>GPMPGEIRPTIGQQMETGDQRFGDLVFRQLAPNVWQHTSYLDMPGFGAVASNGLIVRDGGRVLVVDTAWTDDQTAQILNWIKQEINLPVALAVVTHAHQDKMGGMDALHAAGIATYANALSNQLAPQEGMVAAQHSLTFA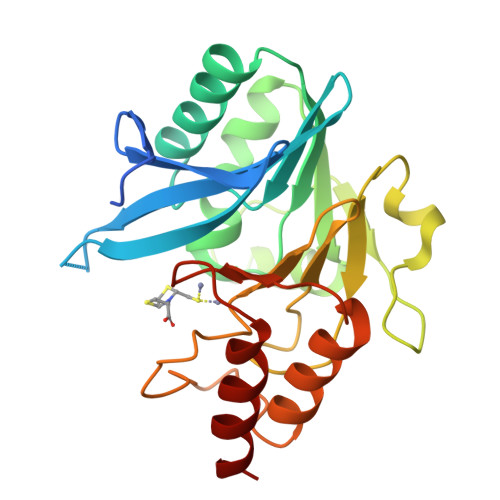ANGWVEPATAPNFGPLKVFYPGPGHTSDNITVGIDGTDIAFGGCLIKDSKAKSLGNLGDADTEHYAASARAFGAAFPKASMIVMSHSAPDSRAAITHTARMADKLR[4x]> GLPV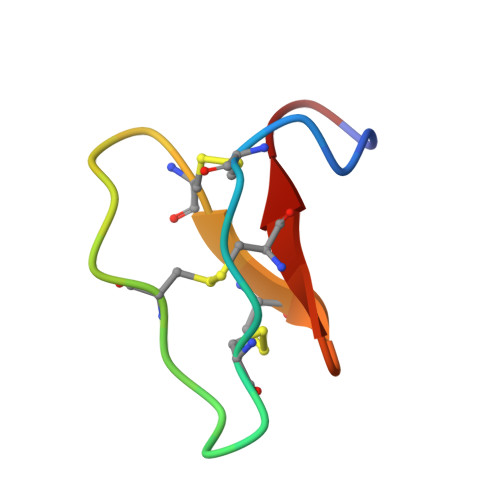CGETCVGGTCNTPGCTCSWPACTRN> MKRQGKRPSKNLKARCSRKALHVNFKDMGWDDWIIAPLEY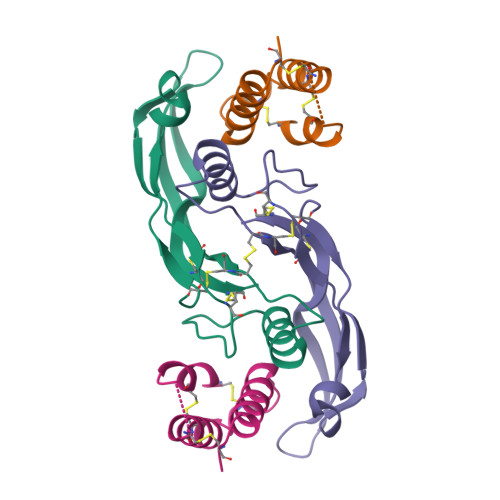EAFHCEGLCEFPLRSHLEPTNHAVIQTLMNSMDPESTPPTCCVPTRLSPISILFIDSANNVVYKQYEDMVVESCGCR;> ETGQCKILRCNAEYVSSTLSLRGGGSSGALRGGGGGGRGGGVGSGGLCRALRSYALCTRRTARTCRGDLAFHSAVHGIEDLMIQHNCSRQGPTAPPPPRGPALPGAGSGLPAPGTKHHHHHH The Ca2+ influx is mediated by MCU, driven by membrane potential and using a uniporter mechanism. Patch-clamp analysis of MCU currents demonstrated that MCU is a channel with exceptionally high Ca2+ selectivity. The MCU subunit comprises three structural domains: the transmembrane domain (TMD), the coiled-coil domain (CCD), and the N-terminal domain (NTD). The TMD of MCU is known to be responsible for Ca2+ selectivity and conduction, and each MCU subunit contributes two transmembrane helices to the TMD: TM1 and TM2.

In conclusion, here we report the structure of intact MCU supercomplex as a 20-subunit O-shaped dimer of hetero-decamers, with auxiliary MICU1 and MICU2 subunits attached. MEMMS has a molecular weight of about 480 kDa and an overall dimension of 210 Å × 190 Å. The overall structure forms an O-shaped ring and adopts the shape like that of two “goldfish”, as if glued together at both their heads (MICU1/MICU2 dimer) and tails (NTD of MCU). A pair of MICU1-MICU2 heterodimer appears like a bridge across the gap between the two halves of MCU-EMRE complex. Within the MEMMS structure, we modelled 2 Ca2+ ions at the E264 sites (MCU has high affinity for Ca2+ (≤2 nmol/L), E264 site is constitutively bound to Ca2+ under physiological conditions), 8 cardiolipins (CDLs), and 16 phosphatidylcholines (PCs). There is no direct interaction between MICU1 and MCU. MICU1 and MICU2 form a heterodimer in a previously reported “face-to-face” pattern, while the two MICU2 subunits interact in a ‘back-to-back’ pattern. The negatively charged C-terminal loops of EMRE protrude into the IMS and are responsible for direct interaction with MICU1. The positively charged N-terminal poly-K (99–102) region of MICU1 and the negatively charged C-terminal tail (93–107) of EMRE are in close proximity to each other, as shown by clear interactions between MICU1 G105, F106 and EMRE E93, E101, consistent with a previous functional study which has detected interactions between these two oppositely charged tails. To conclude, the N-terminal domain and SKK sequence of MICU1 are important for its recruitment onto MCU/EMRE complex through interactions with the C-terminal tails of two adjacent EMRE subunits.

>[8x]DDVTVVYQNGLPVISVRLPSRRERCQFTLKPISDSVGVFLRQLQEEDRGIDRVAIYSPDGVRVAASTGIDLLLLDDFKLVINDLTYHVRPPKRDLLSHENAATLNDVKTLVQQLYTTLCIEQHQLNKERELIERLEDLKEQLAPLEKVRIEISRKAEKRTTLVLWGGLAYMATQFGILARLTWWEYSWDIMEPVTYFITYGSAMAMYAYFVMTRQEYVYPEARDRQYLLFFHKGAKKSRFDLEKYNQLKDAIAQAEMDLKRLRDPLQVHLPLRQIG;>[8x]VIVTRSGAILPKPVKMSFGLLRVFSIVIPFLYVGTLISKNFAALLEEHDIFVPE;>MFRLNSLSALAELAVGSRWYHGGSQPIQIRRRLMMVAFLGASAVTASTGLLWKRAHAESPPCVDNLKSDIGDKGKNKDEGDVCNHEKKTADLAPHPEEKKKKRSGFRDRKVMEYENRIRAYSTPDKIFRYFATLKVISEPGEAEVFMTPEDFVRSITPNEKQPEHLGLDQYIIKRFDGKKISQEREKFADEGSIFYTLGECGLISFSDYIFLTTVLSTPQRNFEIAFKMFDLNGDGEVDMEEFEQVQSIIRSQTSMGMRHRDRPTTGNTLKSGLCSALTTYFFGADLKGKLTIKNFLEFQRKLQHDVLKLEFERHDPVDGRITERQFGGMLLAYSGVQSKKLTAMQRQLKKHFKEGKGLTFQEVENFFTFLKNINDVDTALSFYHMAGASLDKVTMQQVARTVAKVELSDHVCDVVFALFDCDGNGELSNKEFVSIMKQRLMRGLEKPKDMGFTRLMQAMWKCAQETAWDFALPKQ[2x];>PSLRKQRFMQFSSLEHEGEYYMTPRDFLFSVMFEQMERKTSVKKLTKKDIEDTLSGIQTAGCGSTFFRDLGDKGLISYTEYLFLLTILTKPHSGFHVAFKMLDTDGNEMIEKREFFKLQKIISKQDDLMTVKTNETGYQEAIVKEPEINTTLQMRFFGKRGQRKLHYKEFRRFMENLQTEIQEMEFLQFSKGLSFMRKEDFAEWLLFFTNTENKDIYWKNVREKLSAGESISLDEFKSFCHFTTHLEDFAIAMQMFSLAHRPVRLAEFKRAVKVATGQELSNNILDTVFKIFDLDGDECLSHEEFLGVLKNRMHRGLWVPQHQSIQEYWKCVKKES[2x]>[2x]MGSDKIHHHHHHENLYF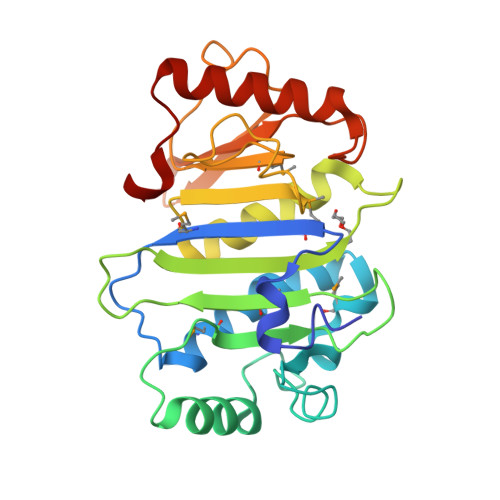QGMEIKAMFRDVSLSSRNFSEMLSRESKVVAALAAKSPLMAHANWRLKGNSLEEATLYPAFDADGSPSTPALAVLNEEQRGKKHSASHAAIWNGNTRPNEGASMSCHVSDEKVLPDRFSTRLGVPDCYAKSQDLADVVTTIVAAFNPLVVEASPEGYFDKQVFDDKPGVGWMLYLPKVITQQQVPEARALIPVSAKGKQTGTIIVSVTDAPFSVDNPEHVAIANRIEIRLVDQDLLPAYVDI>CMKWDYGEMEDFSVSASGLFITNEGNFQYSNATLSYYDPATCEVENEVFYRANGFKLGDVAQSMVIRDGIGWIVVNNSHVIFAIDINTFKEVGRITGFTSPRYIHFLSDEKAYVTQIWDYRIFIINPKTYEITGYIECPDMDMESGSTEQMVQYGKYVYVNCWSYQNRILKIDTETDKVVDELTIGIQPTSLVMDKYNKMWTITDGGYEGSPYGYEAPSLYRIDAETFTVEKQFKFKLGDWPSEVQLNGTRDTLYWINNDIWRMPVEADRVPVRPFLEFRDTKYYGLTVNPNNGEVYVADAIDYQQQGIVYRYSPQGKLIDEFYVGIIPGAFCWKLEHHHHHH[2x]

Contrasting with Enterobacteria, members of the dominant genus Bacteroides often encode several BtuB vitamin B12 outer membrane transporters together with a conserved array of surface-exposed B12-binding lipoproteins. Here we show that the BtuB transporters from Bacteroides thetaiotaomicron form stable, pedal bin-like complexes with surface-exposed BtuG lipoprotein lids, which bind B12 with high affinities. Closing of the BtuG lid following B12 capture causes destabilisation of the bound B12 by a conserved BtuB extracellular loop, causing translocation of the vitamin to BtuB and subsequent transport. We propose that TonB-dependent, lipoprotein-assisted small molecule uptake is a general feature of Bacteroides spp. that is important for the success of this genus in colonising the human gut.

Here we present X-ray crystal structures of B. theta BtuG2 complexed with cyanocobalamin (the manufactured and most stable form of B12, CNCbl), adenosylcobalamin (one of the biologically active forms of vitamin B12 with the bulkiest upper ligand, AdoCbl) as well as the precursor cobinamide (Cbi), which lacks the lower ligand and the nucleotide loop. The cavity that contains the cyano upper ligand is narrowed by Trp194, Trp272 and Tyr316 (numbering based on the annotated Uniprot sequence, including the signal peptide). To explore if this narrow pocket could accommodate a cobalamin with a bulky upper ligand, we obtained a structure to 2.3 Å resolution of BtuG2 co-crystallised with AdoCbl. In this structure the side chain of Trp272 has rotated, enlarging the cavity to fit the adenosyl group. The interaction is stabilised by stacking forces from Trp272 and a hydrogen bond between the hydroxyl group of Tyr335 and the nitrogen in position 3 of the pyrimidine ring of the adenosyl group. For both structures the hydrogen bonds interacting with the side chains of the corrin ring are identical. Thus, given that the lower ligand does not interact with the protein, the structures suggest that BtuG2 can bind many different, if not all, corrinoids.> MSPRKTYILK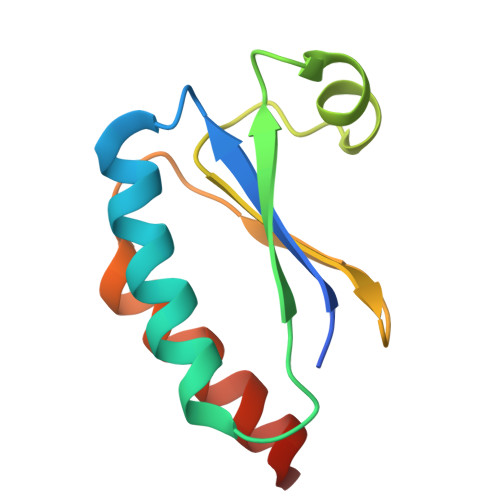LYVAGNTPNSVRALKTLKNILEVEFQGVYALKVIDVLKNPQLAEEDKILATPTLAKVLPLPVRRIIGDLSDREKVLIGLDLLYGELQDSDDF>[2x]EKEMIERDMREYRGFSRAVRAVFEEKERFPGLVDVVSNL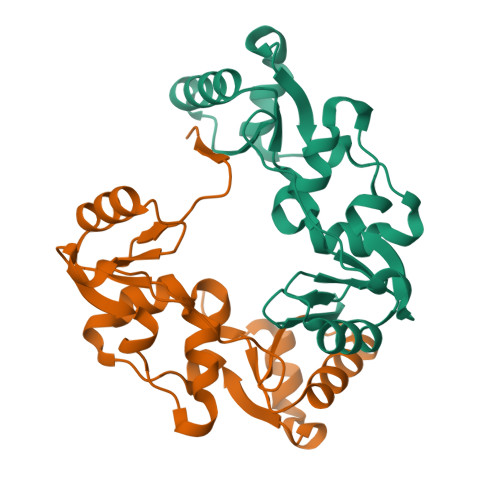IEVDEKYSLAVSVLLGGTAQNIVVRNVDTAKAIVEFLKQNEAGRVTILPLDLIDGSFNRISGLENERGFVGYAVDLVKFPSDLEVLGGFLFGNSVVVETLDDAIRMKKKYRLNTRIATLDGELISGRGAITGGREERSSNVFERRIK> GSA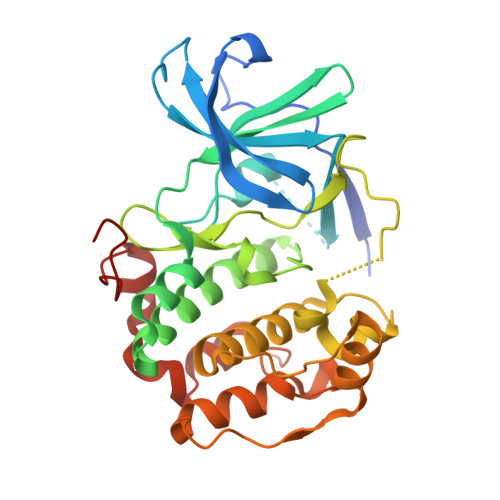SNPQTEEVSIKEIAITHHVKEGHEKADPSQFELLKVLGQGSFGKVFLVKKISGSDARQLYAMKVLKKATLKVRDRVRTKMERDILVEVNHPFIVKLHYAFQTEGKLYLILDFLRGGDLFTRLSKEVMFTEEDVKFYLAELALALDHLHSLGIIYRDLKPENILLDEEGHIKLTDFGLSKESIDHEKKAYSFCGTVEYMAPEVVNRRGHTQSADWWSFGVLMFEMLTGTLPFQGKDRKETMTMILKAKLGMPQFLSPEAQSLLRMLFKRNPANRLGAGPDGVEEIKRHSFFSTIDWNKLYRREIHPPFKPATGRP> RKIIHVDMDCFFAAVEMRDNPALRDIPIAIGGSRERRGVISTANYPARKFGVRSAMPTGMALKLCPHLTLLPGRFDAYKEASNHIREIFSRYTSRIEPLSLDEAYLDVTDSVHCHGSATLIAQEIRQTIFNELQLTASAGVAPVKFLAKIASDMNKPNGQFVITPAEVPAFLQTLPLAKIPGVGKVSAAKLEAMGLRTCGDVQKCDLVMLLKRFGKFGRILWERSQGIDERDVNSERLRKSVGVERTMAEDIHHWSECEAIIER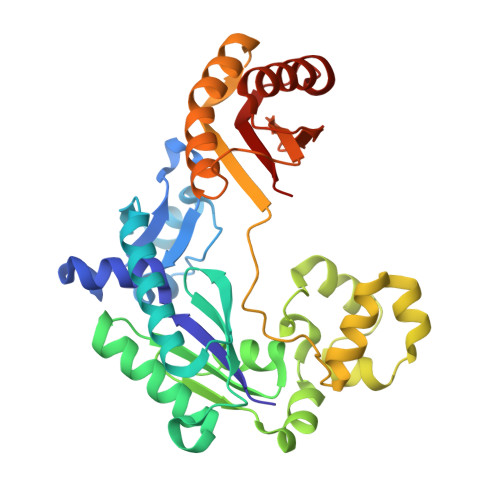LYPELERRLAKVKPDLLIARQGVKLKFDDFQQTTQEHVWPRLNKADLIATARKTWDERRGGRGVRLVGLHVTLD> GHMSKKELAAQIAEKFTDVLSKTHAEE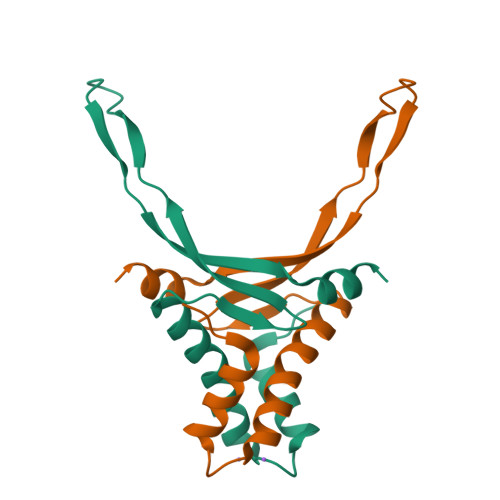ITNFVFDHIKKALVAGKEVSIAGFGKFAVTERAARDGRNPSTGETIKIPASKSAKFKAGKQLKTDLNNN> TD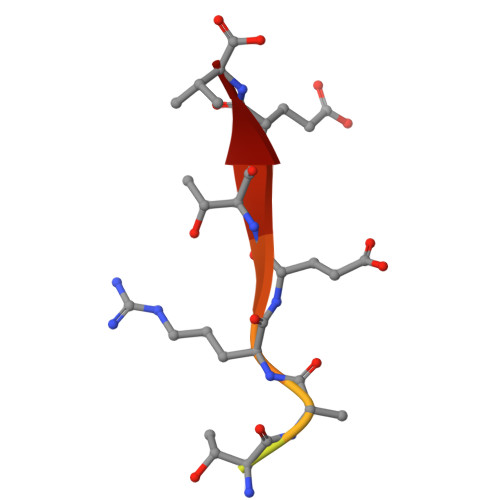DSKPTRRETEV> MATDVAQGPNGRALAESMNPDLLSAIQQHISIERYASVTYLAMSIWCAE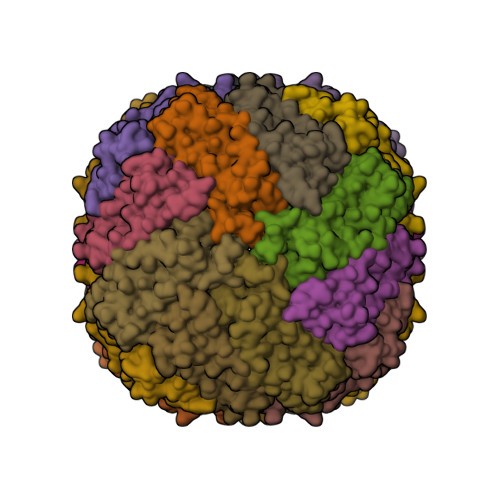RELAGFYQFFDGEAKDEQSHAVHFTQYLIARSQSNDLQTLDAPRQNWDSLASLMATAFQMEADTTSSIQSVYALAERNSDTRTTVFLAPLIEAQIQSEDQFAYLLGRVKFANGDPTALLVIDNELRAGQTQRG>[4x]MAGETVITVVGNLVDDPELRFTPSGAAVAKFRVASTPRTFDRQTNEWKDGESLFLTCSVWRQAAENVAESLQRGMRVIVQGRLKQRSYEDREGVKRTVYELDVDEVGASL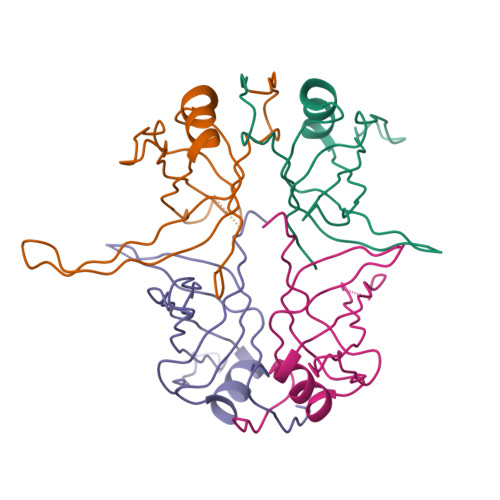RSATAKVTKTSGQGRGGQGGYGGGGGGQGGGGWGGGPGGGQQGGGAPADDPWATGGAPAGGQQGGGGQGGGGWGGGSGGGGGYSDEPPF5-METHYL-3-PHENYL-1H-PYRAZOLE | C10 H10 N2 | 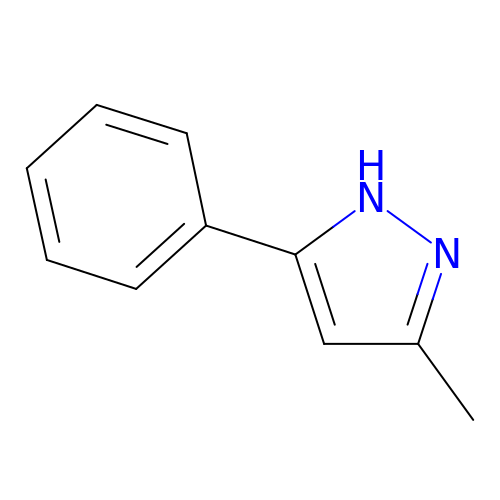QHRSESMSOJZMCO-UHFFFAOYSA-N> A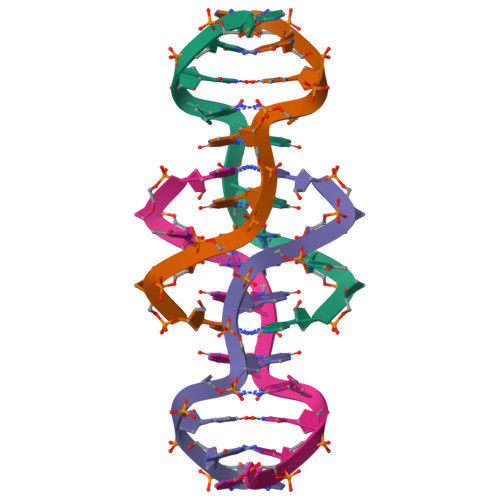CTCGGATGAT> SHIEGYECQPIFLNVLEAIEPGVVCAGHDNNQPDSFAALHSSLNELGERQLVHVVKWAKALPGFRNLHVDDQMAVIQYSWMGLMVFAMGWRSFTNVNSRMLYFAPDLVFNEYRMHKSRMYSQCVRMRHLSQEFGWLQITPQEFLCMKALLLFSIIPVDGLKNQKFFDELRMNYIKELDRIIACKRKNPTSCSRRFYQLTKLLDSVQPIARELYQLAFDLLIKSHMVSVDFPEMMAEIISVQVPKILSGKVKPIYFH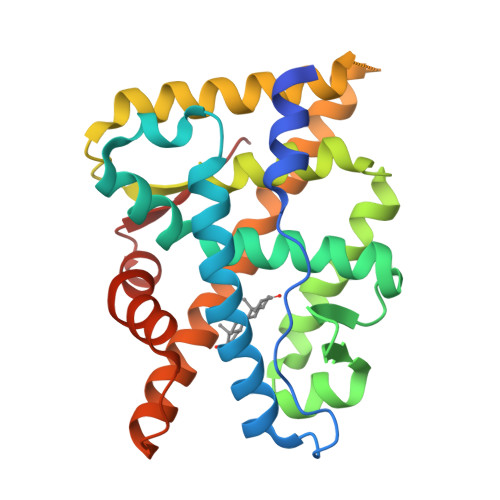TQ>MNIQKSENKANPQKLVVALLPDESAATVIQNNKGLEMYLENKLNKDIELFVSTDYSSMIEVASKGRLDLAYFGPLSYVLAKTKSNIEPFAALEKDGKNTYQALVIGNAEAGINSYEKIEGKIMAYGDQASTSS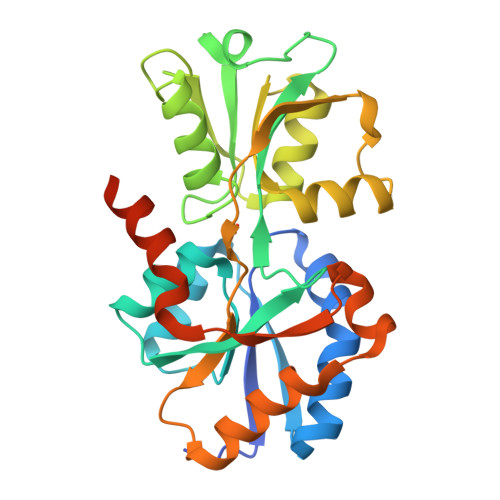HLIPKSMLKQKQLKAGENYEEVFVGAHDAVAIAVANGKAQAGGLSKPIFTALIERGTIDKNKVIIIAESKPFPQYPWTMRSDLDSELKTQIQQAFLELEDKAILKPFKADAFTLVTDQDYDVVRNLGEVLELNFEQLNKLEHHHHHH[2x]>MSLKKLRIGVVGLGGIAQKAWLPVLAAASDWTLQGAWSPTRAKALPICESWRIPYADSLSSLAASCDAVFVHSSTASHFDVVSTLLNAGVHVCVDKPLAENLRDAERLVELAARKKLTLMVGFNRRFAPLYGELKTQLATAASLRMDKHRSNSVGPHDLYF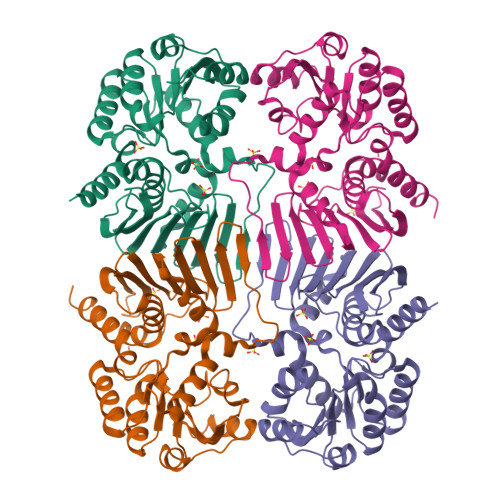TLLDDYLHVVDTALWLSGGKASLDGGTLLTNDAGEMLFAEHHFSAGPLQITTCMHRRAGSQRETVQAVTDGALIDITDMREWREERGQGVVHKPIPGWQSTLEQRGFVGCARHFIECVQNQTVPQTAGEQAVLAQRIVDKIWRDAMSEEGGSHHHHHH[2x]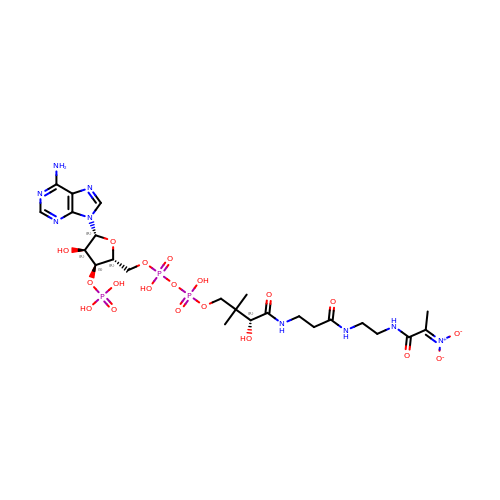[1-[2-[3-[[(2~{R})-4-[[[(2~{R},3~{S},4~{R},5~{R})-5-(6-aminopurin-9-yl)-4-oxidanyl-3-phosphonooxy-oxolan-2-yl]methoxy-oxidanyl-phosphoryl]oxy-oxidanyl-phosphoryl]oxy-3,3-dimethyl-2-oxidanyl-butanoyl]amino]propanoylamino]ethylamino]-1-oxidanylidene-propan-2-ylidene]-bis(oxidanidyl)azanium | C24 H39 N9 O19 P3 | NCNYDGGYTDSUKJ-CUDSEXNASA-N> MTTPVVANYENASMAADYIKRVSNVLPDIGIICGSGLGKLIEEIEERKVIPYINIPNFPKTTVAGHVGNLVLGSVGGRKIVAMQGRLHMYEGYSNQEIALP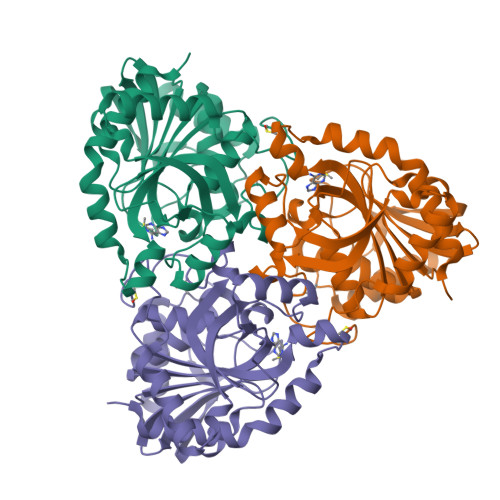IRVMKLLGVRVLLITNLAGGINRKLKSGDFVLIKGHINFPGLGLNNVLVGPNQDEFGPRFPDLSNAYDRLLQQLALKIAQENDFQDLVHEGVYAFNGGPTYESPDESNMLLKLGCDVVGMSTVPEVIIACHCGIKVLAVSLIANNSILDAENDVSINHEKVLAVAEKRADLLQMWFKEIITRLPLD> QENQDGRYSLTYIYTGLSKHVEDVPAFQALGSLNDLQFFRYNSKDRKSQPMGLWRQVEGMEDWKQDSQLQKAREDIFMETLKDIVEYYNDSNGSHVLQGRFGCEIENNRSSGAFWKYYYDGK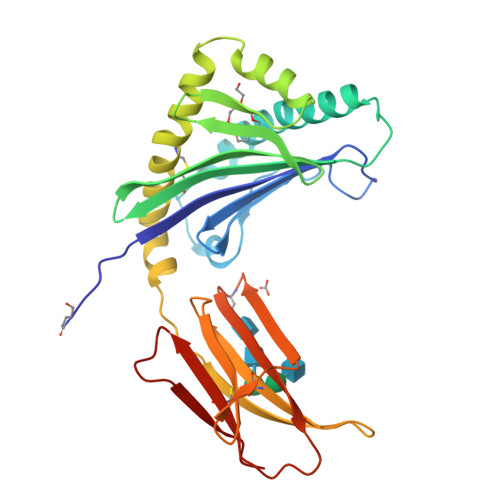DYIEFNKEIPAWVPFDPAAQITKQKWEAEPVYVQRAKAYLEEECPATLRKYLKYSKNILDRQDPPSVVVTSHQAPGEKKKLKCLAYDFYPGKIDVHWTRAGEVQEPELRGDVLHNGNGTYQSWVVVAVPPQDTAPYSCHVQHSSLAQPLVVPWEAS;> QDNTRKIIIKNFDIPKSVRPNDEVTAVLAVQTELKECMVVKTYLISSIPLQGAFNYKYTACLCDDNPKTFYWDFYTNRTVQIAAVVDVIRELGICPDDAAVIPIKNNRFYTIEILKVE> GAYTGVP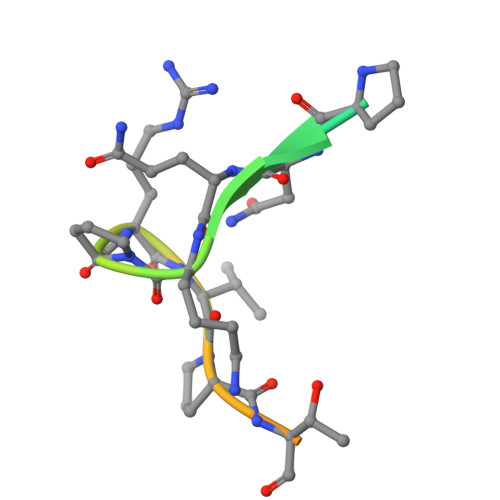NQKPRVPTLRQAKVQ>GPGSMKRVVITGMGGVTALGSRWDEIEAALKAGRNAVRRMPDWDYFESLHTRLAAPLPGFAQPADWPRKKTRSMGRVSMYAVRASELALADAGFAGDESISDGRMGVAYGSSSGSVEPIRAFGTMLESGSMTDVTSNSYVQMMPHTTAVNVSLFWDLKGRIVPTSSACASGSQAIGYAYENIAMGKQTLMLAGGAEELSGPAVAVFDTLYATSTRNDEPHLTPRPFDAKRDGLVVGEGAATLVLEEYEHAKARGATIHAEIVGFGCNSDGAHMTQPTASTMARAMQLALEDAKLDANAIAYVNAHGTSTDRGDVAESQATARTFGERMPISSLKSYVGHTLGACGALEAWWTIEMMKRNWYAPTLNLTEVDPACAPLDYIRGEARAIDAEYVMSNNFAFGGINTSLIFRRV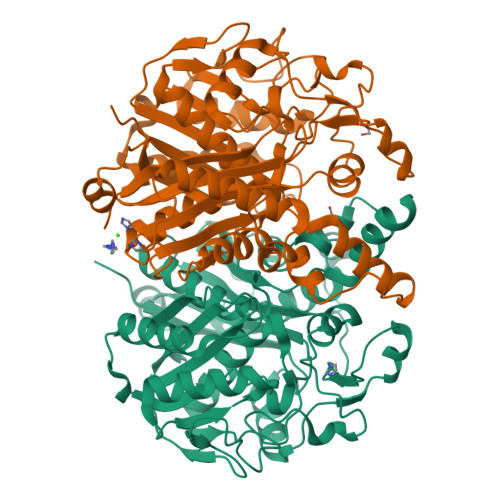R[2x]(SOUTH)-METHANOCARBA-THYMIDINE 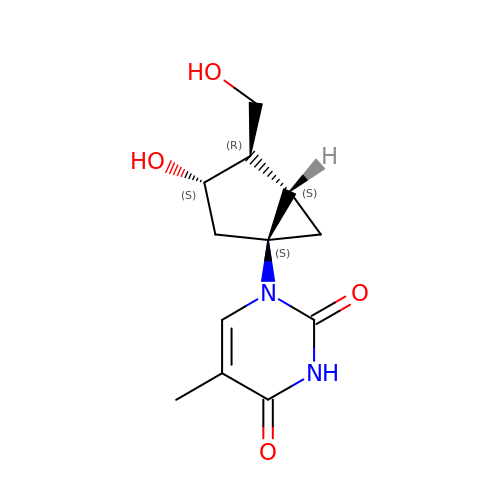| C12 H16 N2 O4 | XRMLXZVSFIBRRJ-PEFMBERDSA-N2-amino-5-(phenylsulfanyl)-3,9-dihydro-4H-pyrimido[4,5-b]indol-4-one | C16 H12 N4 O S | 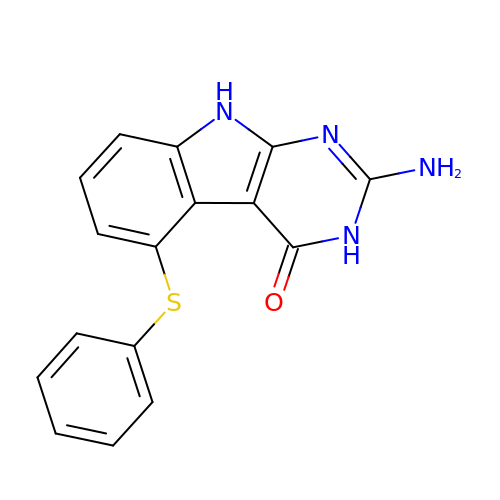RURPYDOTPJEGPP-UHFFFAOYSA-N>MAKRRKIKPMDDEQVLRHLDQLVNDALDFNSSELSKQRSEALKYYFGEPFGNERPGKSGIVSRDVQETVDWIMPSLMKVFTSGGQVVKYEPDTAEDVEQAEQETEYVNYLFMRKNEGFKVMFDWFQDTLMMKTGVVKVYVEEVLKPTFERFSGLSEDMVADILSDPDTSILAQSVDDDGTYTIKIRKDKKKREIKVLCVKPENFLVDRLATCIDDARFLCHREKYTVSDLRLLGVPEDVIEELPYDEYEFSDSQPERLVRDNFDMTGQLQYNSGDDAEANREVWASECYTLLDVDGDGISELRRILYVGDYIISNEPWDCRPFADLNAYRIAHKFHGMSVYDKIRDIQEIRSVLMRNIMDNIYRTNQGRSVVLDGQVNLEDLLTNEAAGIVRVKSMNSITPLETPQLSGEVYGMLDRLEADRGKRTGITDRTRGLDQNTLHSNQAAMSVNQLMTAAEQQIDLIARMFAETGVKRLFQLLHDHAIKYQN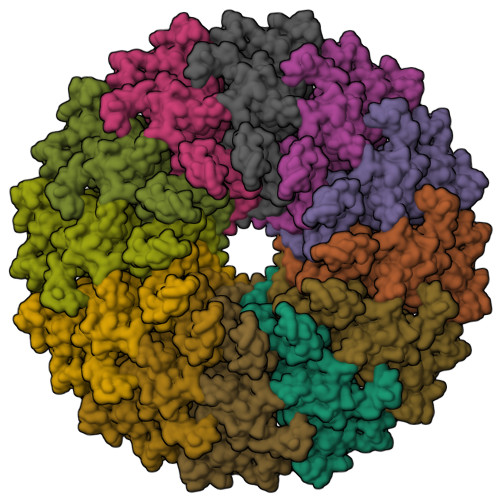QEEVFQLRGKWVAVNPANWRERSDLTVTVGIGNMNKDQQMLHLMRIWEMAQAVVGGGGLGVLVSEQNLYNILKEVTENAGYKDPDRFWTNPNSPEALQAKAIREQKEAQPKPEDIKAQADAQRAQSDALAKQAEAQMKQVEAQIRLAEIELKKQEAVLQQREMALKEAELQLERDRFTWERARNEAEYHLEATQARAAYIGDGKVPETKKPTKAVRR[12x]> NCSKIHLSTKLLAV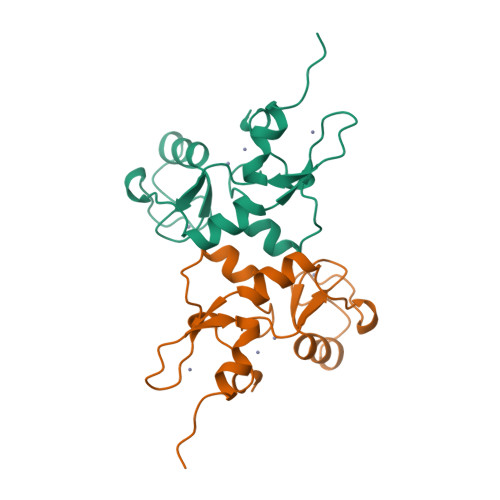DFPAHFVKSISCQICEHILADPVETSCKHLFCRICILRCLKVMGSYCPSCRYPCFPTDLESPVKSFLNILNSLMVKCPAQDCNEEVSLEKYNHHVSSHKESK> MALRGTVTDFSGFDGRADAEVLEKAMKGLGTDEDSILN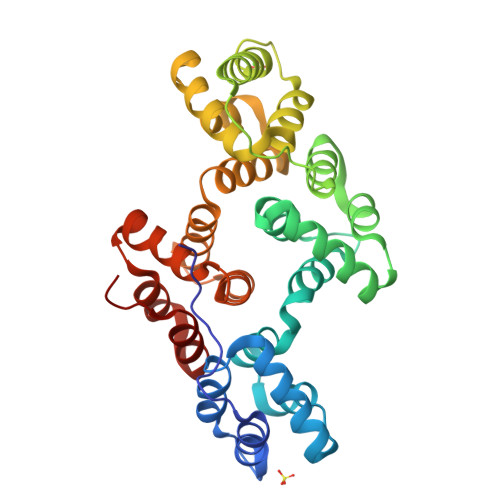LLTARSNAQRQQIAEEFKTLFGRDLVNDMKSELTGKFEKLIVALMKPSRLYDAYELKHALKGAGTDEKVLTEIIASRTPEELRAIKQAYEEEYGSNLEDDVVGDTSGYYQRMLVVLLQANRDPDTAIDDAQVELDAQALFQAGELKWGTDEEKFITILGTRSVSHLRRVFDKYMTISGFQIEETIDRETSGNLENLLLAVVKSIRSIPAYLAETLYYAMKGAGTDDHTLIRVIVSRSEIDLFNIRKEFRKNFATSLYSMIKGDTSGDYKKALLLLCGGEDD> MESKNKTAATQQSEPNVIAAHKGVNQAPVPLKMERVGPHDVHIEMTAQITDIEIDKGKIYKAWTFNGQAPGPLVVVNEGDTIHFTLKNMDPVVPHSMNFHAVHASPSKDFIDVMPNKSGTFTYPANKPGVFMYHCGTKPVLQHIANGMHGVIIVKPKNGYPTDKEVDREYVLIQNEWYKYNDMNDFQNGVPSYVVFSSKALKPGDPNTNGDTFTLKEKPLLAKVGEKIRLYINNVGPNEVSSFHVVGTVFDDVYLDGNPNNHLQGMQTVMLPASGGAVVEFTVTRPGTYPIVTHQFNHAQKGAVAMLKVTETGEDDGTETSGH

Copper-containing nitrite reductases (CuNIRs) catalyze transformation of nitrite to nitric oxide, which has impacts on geochemical, agricultural, and medical health fields. CuNIRs typically have an ∼110 kDa homotrimeric structure, like a Reuleaux triangle. Each protomer contains one type 1 copper (T1Cu) and one type 2 copper (T2Cu) site. The Cys residue forms a peptide-bond bridge (Cys-His bridge) together with one of the His ligands at the T2Cu site to transfer the electron to the catalytic T2Cu site, which is coordinated by three His residues and an axial water molecule.

To further obtain insights into the catalytic intermediates of CuNIR, we performed atomic resolution X-ray crystallography with D98N mutant series of GtNIR in which the Asn residue imitates the protonated state of AspCAT. The structures of D98N without NO2- and C135A/D98N with NO2- were determined at 1.05 and 1.12 Å resolution, respectively. A GK-like conformation of D98N is not observed in the D98N structure without NO2-, which indicates that repulsion between NO2- and Asn98 results in the GK-like conformation.> GMDVNVRGPDGFTPLMIAS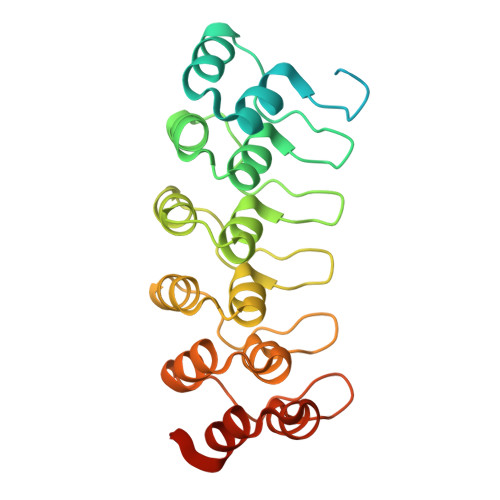CSGGGLETGNSEEEEDAPAVISDFIYQGASLHNQTDRTGETALHLAARYSRSDAAKRLLEASADANIQDNMGRTPLHAAVSADAQGVFQILIRNRATDLDARMHDGTTPLILAARLAVEGMLEDLINSHADVNAVDDLGKSALHWAAAVNNVDAAVVLLKNGANKDMQNNREETPLFLAAREGSYETAKVLLDHFANRDITDHMDRLPRDIAQERMHHDIVRLLDEYNLVRSPQLHG> GPLGSPEFRYFVAMFDY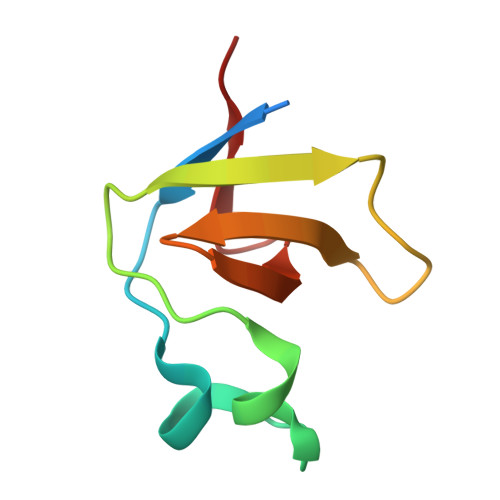DPSTMSPNPDGCDEELPFQEGDTIKVFGDKDADGFYWGELRGRRGYVPHNMVSEVE5-(4-methylpiperazin-1-yl)-2'-(pyridin-2-yl)-1H,1'H-2,5'-bibenzimidazole | C24 H23 N7 | 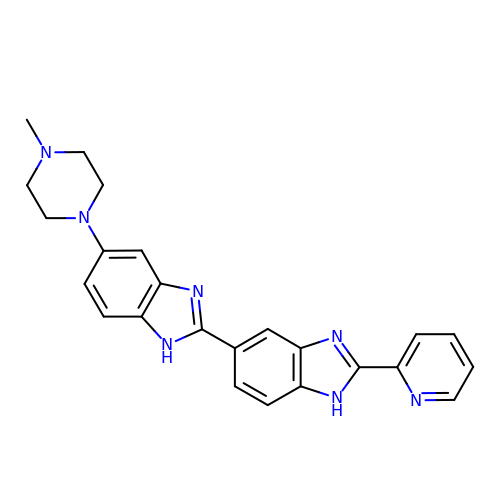QLJMJDOZNAQXQQ-UHFFFAOYSA-N> AGVMTGAKFTQIQFGMTRQQVLDIAGAENCETGGSFGDSIHCRGHAAGDYYAYATFGFTSAAADAKVDSKSQMKLLAPSAPTLTLAKFNQVTVGMTRAQVLATVGQGSCTTWSEYYPAYPSTAG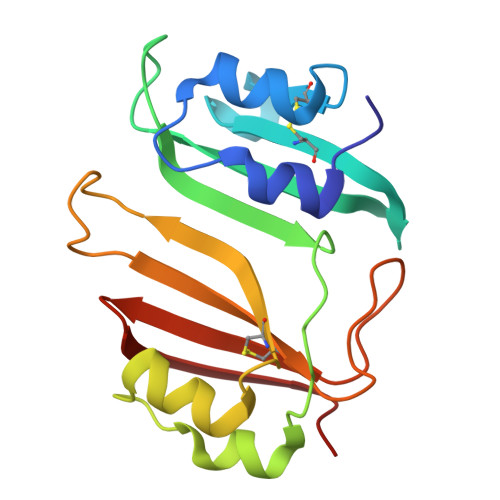VTLSLSCFDVDGYSSTGFYRGSAHLWFTDGVLQGKRQWDLV> MQTTTLNWDTVYAVPINIVNEAIKLKHPTPENFELLNGKYGNCSGSFEEWQITNGGDGSNIRLKIPIKNFKATIIGNRLNGKGGFAFANLEVQVKLKYLPHFPQSKNKDIELVDLKIRTQSDNPEDPAIIVISSYKNIQGFYFEDEYKLTEDDEFVVSYFYRLIKEWLEKNLHFFNYIFNTVNLNLYISDKEKWEWTKPSYVDYAYSEIEGDLSRSALGVLCMTGGRTGSKNQQQKIDPYAIPAASQSGFLISEERLLRNILLPTIPKKFPKSKGDEFEVINESSQGGGYSYILKLKKGKKIDLENIQAVGYTCTPYIQEMKIYLLGSYLKLETTTRVDLPLGVASICETTCEYKFKLSTNNKGEQTIAYEQIGSPVNIQYSENTGNVGLNIVVSFLSATLSF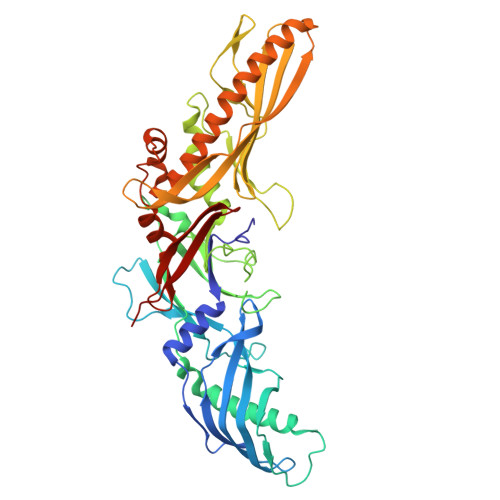ALTFVPGFGTFLAVGLIGGCLIGSVALIPTFIESYNSDTAPSIDLSLENSVSEITWNSSDVFNLDYVALAGPLQLGGTLQVQNS(2,3-dihydro-1H-indol-1-yl)(1H-1,2,3-triazol-1-yl)methanone 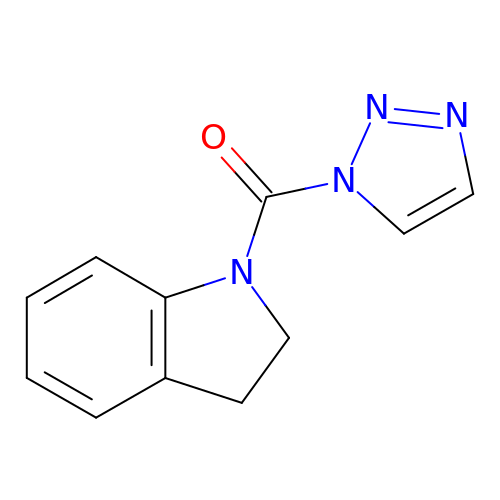| C11 H10 N4 O | YHDLKWQIQYNPEK-UHFFFAOYSA-N> GSHMAFLVQVAADIFNNKVNFELSFPSRPSISELTRSAETAFSNEISLRRPDNVPSHKFHSSKIKMYDEE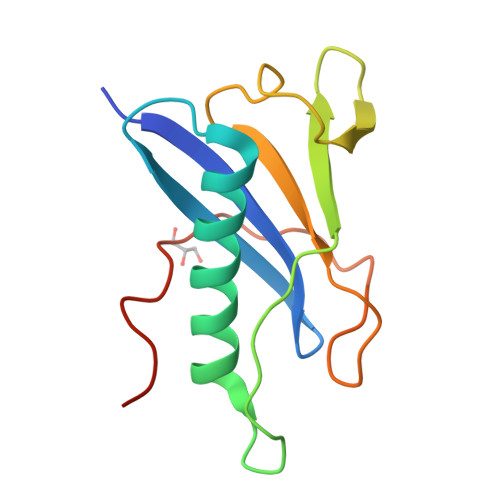LNKWVDLIREDQLTDYCQLYVFQPPNEWHKESQKEIPPAMKPPSSGQRHSAGG> MYEGNNMRSMMGTS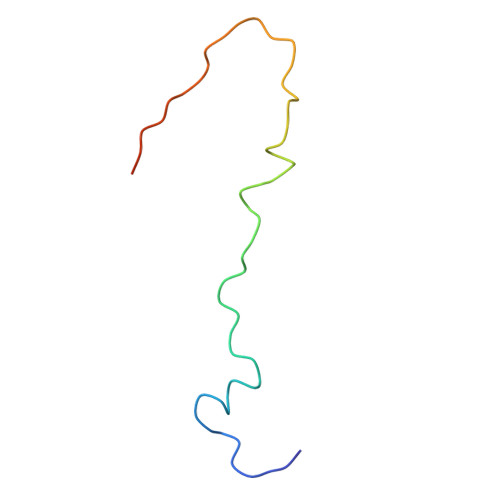YEDSRLNKRTELNENMSIDTNKSEDSYGVQIHSLSKQSFTGDVEEE>[2x]MGHHHHHHSHMGSEIGTGFPFDPHYV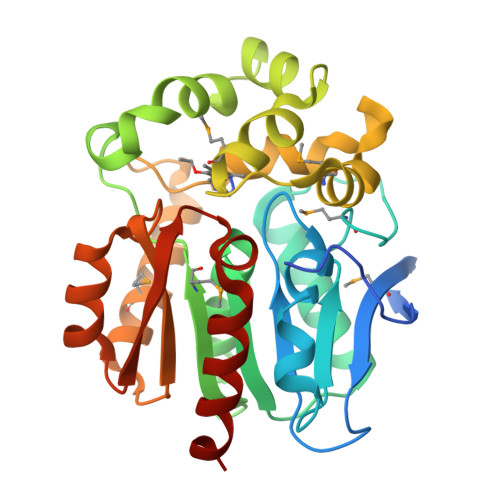EVLGERMHYVDVGPRDGTPVLFLHGNPTSSYLWRNIIPHVAPSHRCIAPDLIGMGKSDKPDLDYFFDDHVRYLDAFIEALGLEEVVLVIHDWGSALGFHWAKRNPERVKGIACMEFIRPIPTWDEWPEFARETFQAFRTADVGRELIIDQNAFIEGALPMGVVRPLTEVEMDHYREPFLKPVDREPLWRFPNELPIAGEPANIVALVEAYMNWLHQSPVPKLLFWGTPGVLIPPAEAARLAESLPNCKTVDIGPGLFLLQEDNPDLIGSEIARWLPGLAG>[2x]STKKKPLTQEQLEDARRLKAIYEKKKNELGLSQESLADKLGMGQSGIGALF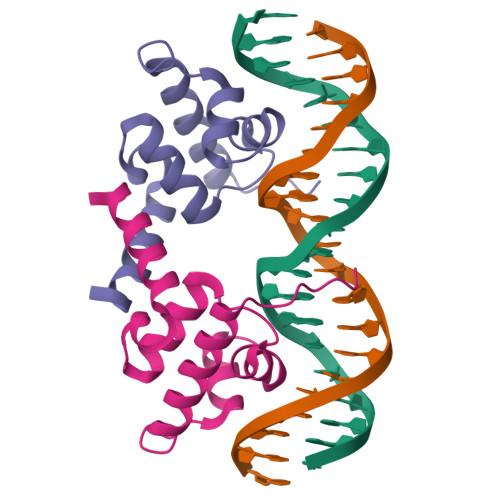NGINALNAYNAALLAKILKVSVEEFSPSIAREIYEMYEAVS>AIATSCHIAEEHIQKVAIFGGTHGNELTGVFLVKHWLENGAEIQRTGLEVKPFITNPRAVKKCTRYIDCDLNRIFDLENLGKKMSEDLPYEVRRAQEINHLFGPKDSEDSYDIIFDLHNTTSNMGCTLILEDSRNNFLIQMFHYIKTSLAPLPCYVYLIEHPSLKYATTRSIAKYPVGIEVGPQPQGVLRADILDQMRKMIKHALDFIHHFNEGKEFPPCAIEVYKIIEKVDYPRDENGEIAAIIHPNLQDQDWKPLHPGDPMFLTLDGKTIPLGGDCTVYPVFVNEAAYYEKKEAFA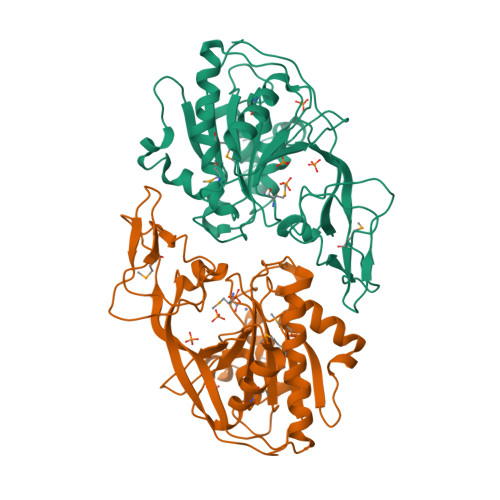KTTKLTLNAKSIRCCLH[2x]Here, we show that T. turnerae encodes a cellulose-active AA10 LPMO. In this context, one of the most significant breakthroughs has been the discovery of chain-breaking “lytic” polysaccharide monooxygenases (LPMOs, sometimes PMOs) that oxidatively deconstruct recalcitrant polysaccharides, most notably cellulose, chitin, hemicelluloses and retrograded starch (generic LPMOs have been extensively reviewed, examples include). When used as part of enzyme cocktails, LPMOs significantly boost the activity of classical glycoside hydrolases, thereby offering great potential for the sustainable breakdown of recalcitrant biomass within a commercial setting. Through mass spectrometry and HPLC analysis of released products, we show that this enzyme has mixed C1–C4 oxidising activity on cellulose and boosts the breakdown of this recalcitrant polysaccharide by glycoside hydrolases.

To gain further insights into the molecular basis for the biochemical properties of TtAA10A, and to probe this, potentially unusual, dual Cu structure, we determined the crystal structure for the recombinantly expressed protein to 1.4 Å resolution. The overall structure revealed a core immunoglobulin-like fold decorated by loops and a helical bundle as typically observed for enzymes from this family. As for all LPMOs studied so far (as defined by their activity), the active site of TtAA10A is formed by the “histidine brace” motif which is located at the centre of an almost flat surface. A single copper ion was modelled at this position coordinated in a typical T-shaped geometry by the amino terminus and side chain of His 1 and the side chain imidazole of His 107. In the axial positions around the active site copper ion, TtAA10A has Phe 195 and Gly 105. It, therefore, appears that the copper in this enzyme has also undergone photo-reduction to the Cu(I) oxidation state. Our structure reveals the position of the second copper-binding site that was observed in the EPR spectra. This site is 14.4 Å (Cu…Cu) from the histidine brace copper ion in a large negatively charged patch on the protein surface. Tyrosine 3 is adjacent (5.3 Å) to the second Cu site, thus providing an efficient charge transfer pathway between the two copper sites.

> HGYIESPPSRQQHCGAEQKPDNPSSAKCDEAFANYRAAGGQNSHWYNFMSVVAHHEGRKVVKGTEHVCGFDGETWNPAPYDTPANWPVTSFNSGQQTFVWDISYGPHFSDTEELVFYITKPGFSFDPTRELTWADFEDQPFCDESIVPGDFSTNSAVEADMANSHINVTCNVPSRSGRHVIFAEWGRNEHTYERFFSCVDVDFGWSHPNFEK Here we investigated water through cryogenic electron microscopy (cryo-EM) on a highly solvated molecule: the Tetrahymena ribozyme. Here we report cryo-EM maps of solvated and enzymatically active Tetrahymena ribozyme without substrate (387 nt, 128 kDa) using cryo-EM in two independent reconstructions at 2.2 Å and 2.3 Å resolution, enabling detailed analysis and confidence estimation of the interactions of ordered water in the context of an intricate RNA tertiary structure. By using segmentation-guided water and ion modelling (SWIM), an approach combining resolvability and chemical parameters, we automatically modelled and cross-validated water molecules and Mg2+ ions in the ribozyme core, revealing the extensive involvement of water in mediating RNA non-canonical interactions. Water is extensively observed in the interior of the ribozyme and can directly mediate interactions between RNA atoms without also coordinating site-bound ions.

To investigate the confidence in their positioning and assignment, we took advantage of the availability of two discrete, independent, high-resolution cryo-EM maps. We examined whether the water modelled in both maps share equivalent locations; shared waters are referred to below as ‘consensus’ waters. Of the SWIM waters, 134 were identified as consensus, 53% and 48% of all SWIM waters in the 2.2 Å and 2.3 Å models, respectively. Although all waters modelled were well resolved (Q > 0.7), consensus waters had a statistically significant higher Q score than non-consensus waters and were in regions of the RNA that were statistically significantly better resolved (higher Q score) and more similar (smaller RMSD). Consensus waters were bound throughout all parts of nucleotides in our cryo-EM structures. Indeed, all resolved tertiary interactions in our structures, which link distant nucleotides in the sequence into stable junctions, were extensively bound to well-positioned waters. For example, the catalytic active site is embedded in a highly conserved core with numerous non-canonical interactions. Stabilizing this core, where the P3 and P6a domains come in close proximity, the Watson–Crick–Franklin edge of C255 and the sugar edge of G272 meet in an orientation that is not favourable for direct hydrogen bonding. We observed an ordered water that bridges these two bases stabilizing the tertiary contact. In the junction between P3 and P7, A306 is adjacent and in the same plane as the A308–U267 base pair, but instead of A306 forming direct RNA–RNA hydrogen bonds with the A–U base pair, the interaction is mediated by two waters.

> GGAGGGAAAAGUUAUCAGGCAUGCACCUGGUAGCUAGUCUUUAAACCAAUAGAUUGCAUCGGUUUAAAAGGCAAGACCGUCAAAUUGCGGGAAAGGGGUCAACAGCCGUUCAGUACCAAGUCUCAGGGGAAACUUUGAGAUGGCCUUGCAAAGGGUAUGGUAAUAAGCUGACGGACAUGGUCCUAACCACGCAGCCAAGUCCUAAGUCAACAGAUCUUCUGUUGAUAUGGAUGCAGUUCACAGACUAAAUGUCGGUCGGGGAAGAUGUAUUCUUCUCAUAAGAUAUAGUCGGACCUCUCCUUAAUGGGAGCUAGCGGAUGAAGUGAUGCAACACUGGAGCCGCUGGGAACUAAUUUGUAUGCGAAAGUAUAUUGAUUAGUUUUGGAG> APECGERA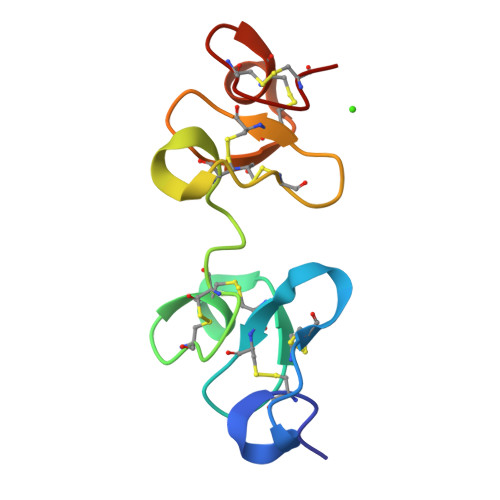SGKRCPNGKCCSQWGYCGTTDNYCGQGCQSQCDYWRCGRDFGGRLCEEDMCCSKYGWCGYSDDHCEDGCQSQCD4-(aminomethyl)-2-{6-[4-(propan-2-yl)-4H-1,2,4-triazol-3-yl]pyridin-2-yl}-2,3-dihydro-1H-isoindol-1-one | C19 H20 N6 O | 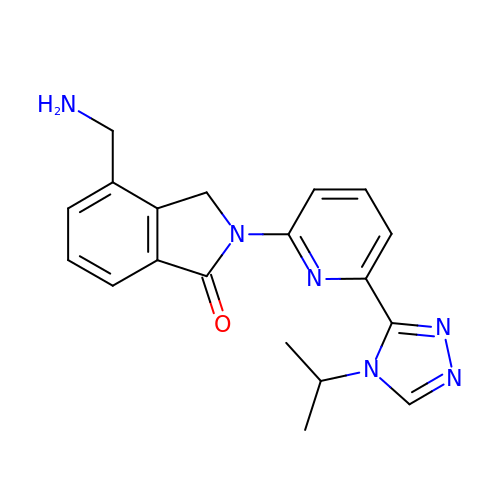BSNVVHMZMJKTCO-UHFFFAOYSA-N> MAPVIPSNTDYPGPHHFEVTFQQSSTAKSATWTYSPLLKKLYCQIAKTCPIQIKVSTPPPPGTAIRAMPVYKKAEHVTDVVKR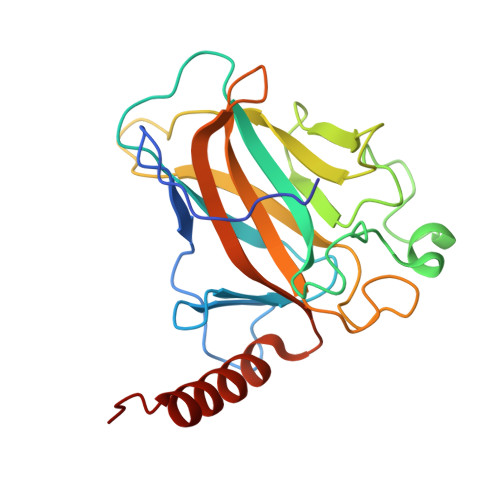CPNHELGRDFNEGQSAPASHLIRVEGNNLSQYVDDPVTGRQSVVVPYEPPQVGTEFTTILYNFMCNSSCVGGMNRRPILIIITLEMRDGQVLGRRSFEGRICACPGRDRKADEDHYREAENLYFQ>MILFRKFRVLILTVFLIACTMHIMIDLLPKLEKRAAGSSSSAGGGSGCSCAHTPGEEPRSWGKQRARAADPGWPNKHSLRLLQDFSNEPNSNLTSQSREKVTERAGSEKQGSGKRGLMREADSRQRRTDVRVSSVLQSLFEHPLYRTVLPDLTEEDTLFNLNAEIRLYPKAAGQQEWHNEGNVEEEEFSPPGEANSESYPNWLRFHIGINRYELYSRHNPVIAALLRDLLSQKISSVGMKSGGTQLKLIMSFQNYGQALFKPMKQTREQETPPDFFYFSDFERHNAEIAAFHLDRILDFRRVPPVAGRLVNMTREIRDVTRDKKLWRTFFVSPANNICFYGECSYYCSTEHALCGKPDQIEGSLAAFLPDLALAKRKTWRNPWRRSYHKRKKAEWEVDPDYCDEVKQTPPYDRGTRLLDIMDMTIFDFLMGNMDRHHYETFEKFGNDTFIIHLDNGRGFGKHSHDEMSILVPLTQCCRVKRSTYLRLQLLAKEEYKLSSLMEESLLQDRLVPVLIK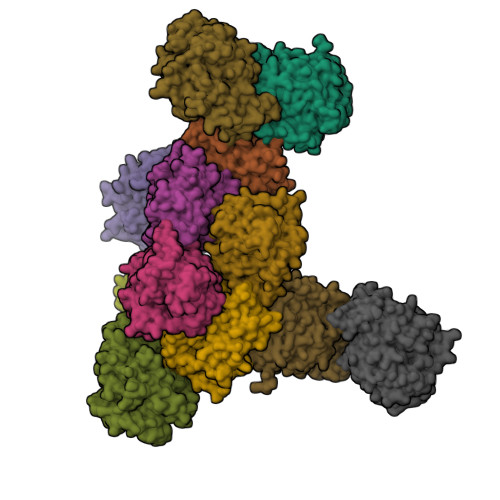PHLEALDRRLRLVLKVLSDCVEKDGFSAVVENDLDGQPSVHGGR[12x]>[2x]MANDSPAKSLVDIDLSSLRDPAGIFELVEVVGNGTYGQVYKGRHVKTGQLAAIKVMDVTEDEEEEIKLEINMLKKYSHHRNIATYYGAFIKKSPPGHDDQLWLVMEFCGAGSITDLVKNTKGNTLKEDWIAYISREILRGLAHLHIHHVIHRDIKGQNVLLT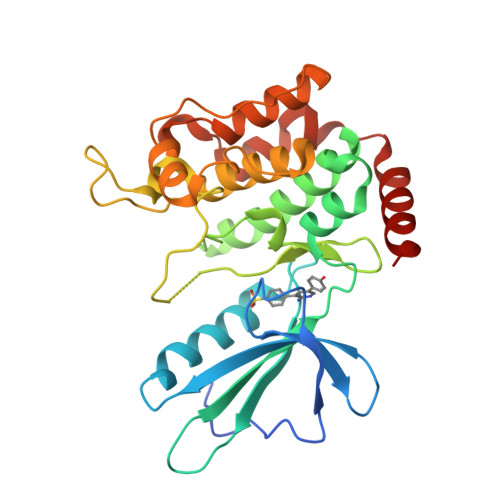ENAEVKLVDFGVSAQLDRTVGRRNTFIGTPYWMAPEVIACDENPDATYDYRSDLWSCGITAIEMAEGAPPLCDMHPMRALFLIPRNPPPRLKSKKWSKKFFSFIEGCLVKNYMQRPSTEQLLKHPFIRDQPNERQVRIQLKDHIDRTR>[6x]PPGPPGPPGPPGPTGP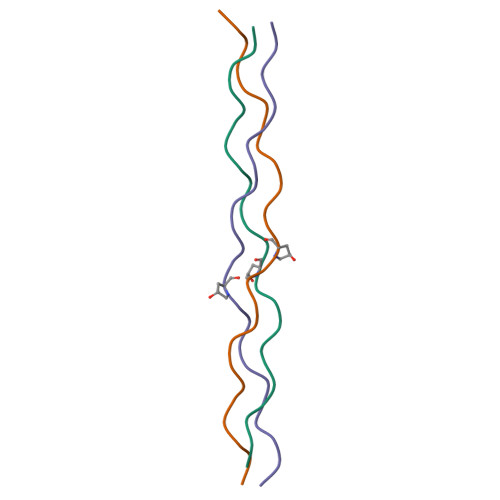PGPPGPPGPPG4-hydroxy-2-oxoglutarate (HOG) aldolase is a unique enzyme in the hydroxyproline degradation pathway catalyzing the cleavage of HOG to pyruvate and glyoxylate. The crystal structures of the apoenzyme and pyruvate-Schiff base intermediate complex are the first for any HOGA enzyme to date and reveal a tetrameric structure composed of a dimer of dimers as well as the identity of active site residues. As mentioned briefly above, the crystallographic symmetry of the hHOGA crystals generate a tetrameric assembly containing a dimer of dimers. Residues 26–259 form an (α/β)8 TIM barrel domain, while residues 260–327 form a three-helical bundle at the C-terminus.

A 2.5 Å resolution dataset was collected for the native apoenzyme at the National Synchrotron Light Source, beamline X25. The model was refined until the Rwork/free values reached 28.0/29.5%, and then used as a molecular replacement search model to solve the structures of the apoenzyme and the Schiff base adduct with pyruvate. Of the 302 residues in the mature form of hHOGA, 296 were modeled for both structures. No electron density was observed for the first six residues of hHOGA and the three residues remaining from the affinity tag. The final structures for the apoenzyme and Schiff base adduct exhibited Rwork/free values of 21.2/24.6% and 19.6/21.6%, respectively, and were of high overall quality, as indicated by the refinement statistics in Table 1. Interestingly, the packing of hHOGA within the unit cell supports only one molecule in the a.s.u. and a solvent content of 75%. The crystallographic symmetry, however, does generate a tetramer that rotates up the 3-fold screw axis, resulting in large solvent channels. A superposition of the apoenzyme structure with the pyruvate adduct (RMSD  = 0.19 Å for Cα atoms) reveals no significant structural changes to the active site other than a water molecule within hydrogen bonding distance to Lys196.

> GPASGEGKKVDIAGIYPPVTTPFTATAEVDYGKLEENLHKLGTFPFRGFVVQGSNGEFPFLTSSERLEVVSRVRQAMPKNRLLLAGSGCESTQATVEMTVSMAQVGADAAMVVTPCYYRGRMSSAALIHHYTKVADLSPIPVVLYSVPANTGLDLPVDAVVTLSQHPNIVGMKDSGGDVTRIGLIVHKTRKQDFQVLAGSAGFLMASYALGAVGGVCALANVLGAQVCQLERLCCTGQWEDAQKLQHRLIEPNAAVTRRFGIPGLKKIMDWFGYYGGPCRAPLQELSPAEEEALRMDFTSNGWL>[2x]SSLDDKPQFPGASAEFIDKLEFIQPNVISGIPIYRVMDRQGQIINPSEDPHLPKEKVLKLYKSMTLLNTMDRILYESQRQGRISFYMTNYGEEGTHVGSAAALDNTDLVFGQYREAGVLMYRDYPLELFMAQCYGNISDLGKGRQMPVHYGCKERHFVTISSPLATQIPQAVGAAYAAKRANANRVVICYFGEGAASEGDAHAGFNFAATLECPIIFFCRN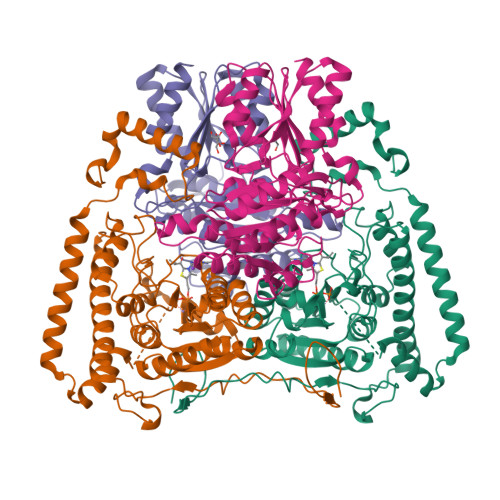NGYAISTPTSEQYRGDGIAARGPGYGIMSIRVDGNDVFAVYNATKEARRRAVAENQPFLIEAMTYRIGHHSTSDDSSAYRPVDEVNYWDKQDHPISRLRHYLLSQGWWDEEQEKAWRKQSRRKVMEAFEQAERKPKPNPNLLFSDVYQEMPAQLRKQQESLARHLQTYGEHYPLDHFDK;>[2x]VAHFTFQPDPEPREYGQTQKMNLFQSVTSALDNSLAKDPTAVIFGEDVAFGGVFRCTVGLRDKYGKDRVFNTPLCEQGIVGFGIGIAVTGATAIAEIQFADYIFPAFDQIVNEAAKYRYRSGDLFNCGSLTIRSPWGCVGHGALYHSQSPEAFFAHCPGIKVVIPRSPFQAKGLLLSCIEDKNPCIFFEPKILYRAAAEEVPIEPYNIPLSQAEVIQEGSDVTLVAWGTQVHVIREVASMAKEKLGVSCEVIDLRTIIPWDVDTICKSVIKTGRLLISHEAPLTGGFASEISSTVQEECFLNLEAPISRVCGYDTPFPHIFEPFYIPDKWKCYDALRKMINYGGHHHHHH> MSQQVDKIKASYPLFLDQDYKDMLAKKRDGFEEKYPQDKIDEVFQWTTTKEYQELNFQREALTVNPAKACQPLGAVLCALGFEKTMPYVHGSQGCVAYYRSYFNRHFREPVSCVSDSMTEDAAVFGGQQNMKDGLQNCKATYKPDMIAVSTTCMAEVIGDDLNAFINNSKKEGFIPDEFPVPFAHTPSFVGSHVTGWDNMFEGIARYFTLKSMDDKVVGSNKKINIVPGFETYLGNFRVIKRMLSEMGVGYSLLSDPEEVLDTPADGQFRMYAGGTTQEEMKDAPNALNTVLLQPWHLEKTKKFVEGTWKHEVPKLNIPMGLDWTDEFLMKVSEISGQPIPASLTKERGRLVDMMTDSHTWLHGKRFALWGDPDFVMGLVKFLLELGCEPVHILCHNGNKRWKKAVDAILAASPYGKNATVYIGKDLWHLRSLVFTDKPDFMIGNSYGKFIQRDTLHKGKEFEVPLIRIGFPIFDRHHLHRSTTLGYEGAMQILTTL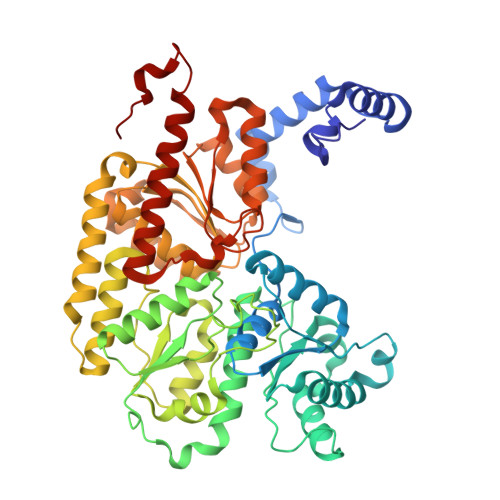VNSILERLDEETRGMQATDYNHDLVR> SLLTEVETYVLSIIPSGPLKAEIAQRLEDVFAGKNTDLEVLMEWLKTRPILSPLTKGILGFVFTLTVPSERGLQRRRFVQNALNGNGDPNNMDKAKKLYRKLKREITFHGAKEISLSYSAGALASCMGLIYNRMGAVTTEVAFGLVCATCEQIADSQHRSHRQMVTTTNPLIRHENRMVLASTTAKAMEQMAGSSEQAAEAMEVASQARQMVQAMRTIGTHPSSSAGLKNDLLENLQAYQKRMGVQMQRFK

The matrix protein M1 is one of the most abundant and most highly conserved proteins of IAV. It is a small, 252-amino–acid protein composed of an α-helical N-terminal domain (NTD) and a C-terminal domain (CTD). Ultrastructural analysis has revealed that the matrix shell within intact virions is formed by a single-helical layer of M1 that is closely associated with the viral membrane. Here, we show that recombinant, soluble full-length M1 from IAV can assemble into 2 different oligomeric forms.

Mutation of V97 to a lysine, predicted to disrupt hydrophobic interactions at either of the C2-symmetry and lateral interfaces observed by crystallography, led to the formation of single-layered oligomers. The M1-V97K oligomers are similar to the matrix layers observed in intact virions, which are also formed by a single-helical layer of M1. We observed relatively straight M1-V97K tubes in vitreous ice and determined a 3.4-Å cryo-EM map. The M1-V97K oligomer is a hollow tube assembled from approximately 21 asymmetric units per helical turn, with inner and outer diameters of 124 Å and 248 Å and a helical pitch of 42 Å. The structure of its NTD contains 9 α-helices (α1–α9) and is identical to the previously solved crystal structure. The CTD forms a helical bundle comprising 3 α-helices (α10–α12) that connect to the NTD within the same molecule via extended connecting loop 9 (CL9). Individual M1-V97K proteins are assembled with their NTDs skewed toward the outside and their CTDs toward the inside of the helical tube. Within each strand, M1 subunits interact via the stacked interface observed in the crystal structures of NTDM1. Interactions between the strands are formed between the CTDs of the lower strand and NTDs of the strand above: for example, between the CTD of N and the NTD of N + 23. At the interface of 3 adjacent subunits, all 5 histidine residues found in the M1 sequence form a cluster.> MFLQRPKPYSDESLESFFIRVANKNGYGDVHRFLEATKRFLQDIDHNGYQTFPTDITRINPYSAKNSSSARTASFLKLAQLTFNEPPELLGLAINRTNMKYSPSTSAVVRGAEVFPRSLLRTHSIPCCPLCLRENGYASYLWHFQGYEYCHSHNVPLITTCSCGKEFDYRVSGLKG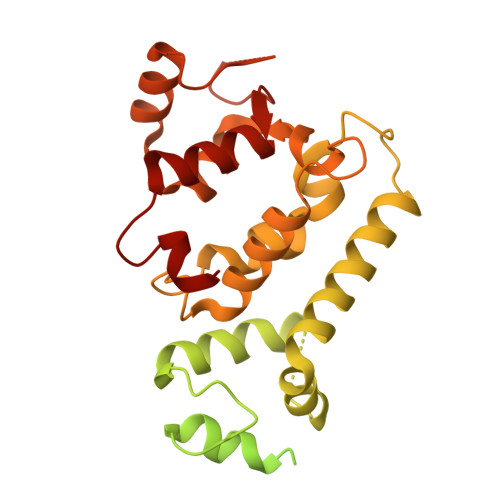ICCKCKEPITLTSRENGHEAACTVSNWLAGHESKPLPNLPKSYRWGLVHWWMGIKDSEFDHFSFVQFFSNWPRSFHSIIEDEVEFNLEHAVVSTSELRLKDLLGRLFFGSIRLPERNLQHNIILGELLCYLENRLWQDKGLIANLKMNALEATVMLNCSLDQIASMVEQRILKPNRKSKPNSPLDVTDYLFHFGDIFCLWLAEFQSDEFNRSFYVSRW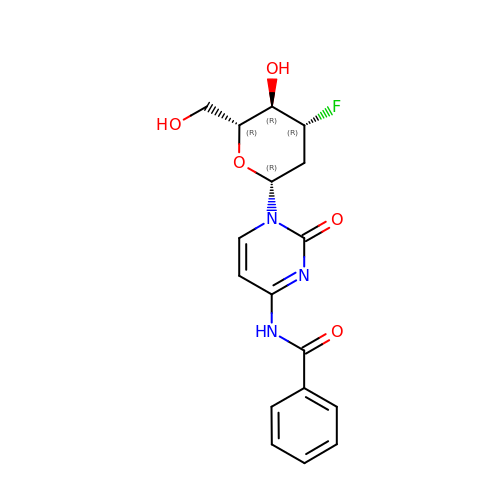1-(2,3-dideoxy-3-fluoro-beta-D-arabino-hexopyranosyl)-4-[(phenylcarbonyl)amino]pyrimidin-2(1H)-one | C17 H18 F N3 O5 | JDMVJAAWOFCRPK-GBOPCIDUSA-N>[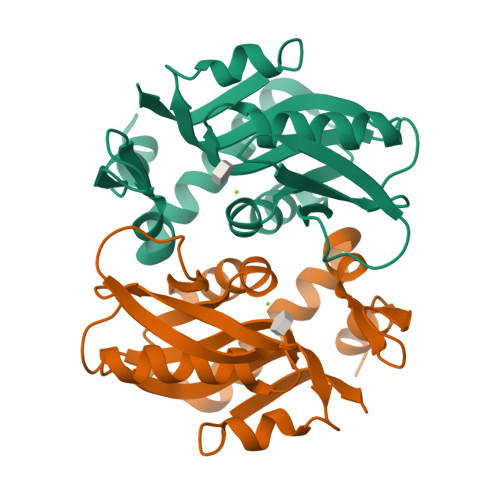2x]DSELQLVEQRIRSFPDFPTPGVVFRDISPVLKDPASFRAAIGLLARHLKATHGGRIDYIAGLDSRGFLFGPSLAQELGLGCVLIRKRGKLPGPTLWASYSLEFGKAELEIQKDALEPGQRVVVVDDLLATGGTMNAACELLGRLQAEVLECVSLVELTSLKGREKLAPVPFFSLLQYE> GSHMAKTYDYLFKLLLIGDSGVGKTCVLFRFSEDAFNSTFISTIGIDFKIRTIEL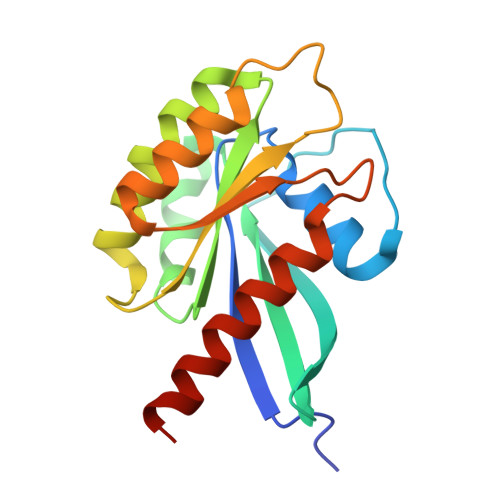DGKRIKLQIWDTAGLERFREITTAYYRGAMGIMLVYDITNEKSFDNIRNWIRNIEEHASADVEKMILGNKCDVNDKRQVSKERGEKLALDYGIKFMETSAKANINVENAFFTLARDIKAKMDKKLEGNS> MSKIFVNPSAIRAGLADLEMAEETVDLINRNIED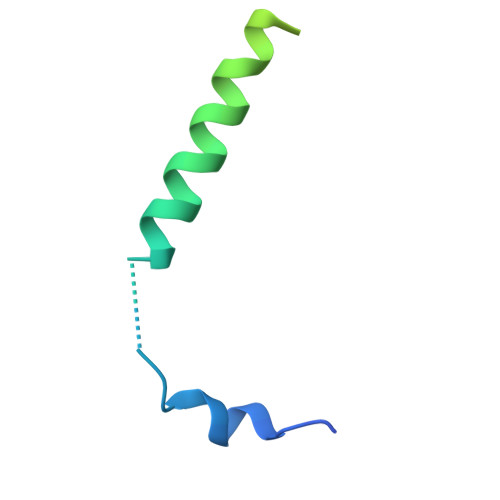NQAHLQGEPIEVDNLPEDMGRLHLDGGKSPNPGELEHHHHHH>[4x]MSQHNEKNPHQHQSPLHDSSEAKPGMDSLAPEDGSHRP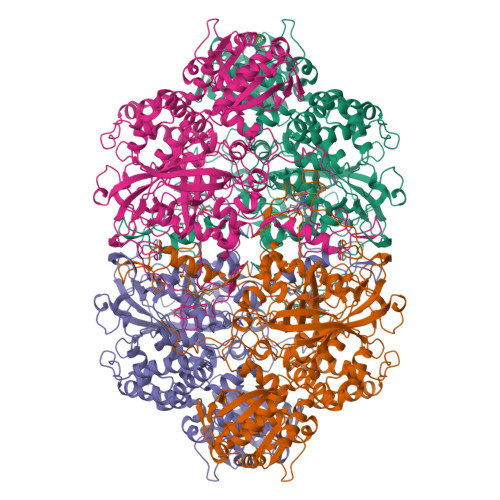AAEPTPPGAQPTAPGSLKAPDTRNEKLNSLEDVRKGSENYALTTNQGVRIADDQNSLRAGSRGPTLLEDFILREKITHFDHERIPERIVHARGSAAHGYFQPYKSLSDITKADFLSDPNKITPVFVRFSTVQGGAGSADTVRDIRGFATKFYTEEGIFDLVGNNTPIFFIQDAHKFPDFVHAVKPEPHWAIPQGQSAHDTFWDYVSLQPETLHNVMWAMSDRGIPRSYRTMEGFGAHTFRLINAEGKATFVRFHWKPLAGKASLVWDEAQKLTGRDPDFHRRELWEAIEAGDFPEYELGFQLIPEEDEFKFDFDLLDPTKLIPEELVPVQRVGKMVLNRNPDNFFAENEQAAFHPGHIVPGLDFTNDPLLQGRLFSYTDTQISRLGGPNFHEIPINRPTCPYHNFQRDGMHRMGIDTNPANYEPNSINDNWPRETPPGPKRGGFESYQERVEGNKVRERSPSFGEYYSHPRLFWLSQTPFEQRHIVDGFSFELSKVVRPYIRERVVDQLAHIDLTLAQAVAKNLGIELTDDQLNITPPPDVNGLKKDPSLSLYAIPDGDVKGRVVAILLNDEVRSADLLAILKALKAKGVHAKLLYSRMGEVTADDGTVLPIAATFAGAPSLTVDAVIVPCGNIADIADNGDANYYLMEAYKHLKPIALAGDARKFKATIKIADQGEEGIVEADSADGSFMDELLTLMAAHRVWSRIPKIDKIPA> MNKTMLKIVAFGVAVIGFYMYITVYVTGLSGTGGGGTATGVSAEAGEQIFWGDGQCSTCHKIGSSGSATRGPDQEGLAERAEERAKELGLSSGLEYLVESIIDPEKYVVEGFDKIMPRVYDPPIMLSREKILAVLAYLQSLGGEPDLDAIMKFKDKIPEASKTKVKPWVPPLAVTAEEGEQVFFDESLDVTCGKCHMVNGKGQKVGPELTGIGAIQTPQYFVESILEPSAVIVKGYETVFVITADGIPYNGLIKSDTEEELTLILEESGSVEEVVIPKDEIEDMKKQEVSICPGNIGELLSVRQFYAVIEYLRSLK

Kustd1711 is a putative electron transfer protein encoded on the nitrite oxidoreductase (nxr) gene cluster of anaerobic ammonium-oxidizing (anammox) bacteria and consists of two heme-containing domains and one additional domain. Here, we describe a diheme cytochrome c with high heme redox potentials of about +350 mV, despite having a large overall negative charge, which typically reduces redox potentials. High-resolution crystal structures, spectroelectrochemical measurements, and high-end computational methods show how this is achieved: each heme iron has a calcium cation positioned next to it at a distance of only 6.9 Å, raising their redox potentials by several hundred millivolts through electrostatic interaction. We suggest that this has evolved to provide the protein with a high redox potential despite its large negative surface charge, which it likely requires for interactions with redox partners.

To improve our confidence in the assignment of the various transitions, we mutated the distal methionine ligands in both the N- and C-terminal heme sites to histidine and cysteine. To confirm that the sites can accommodate these mutations while maintaining six-coordinate heme binding and calcium binding, we determined the crystal structures of the C-terminal domain methionine mutants M292H and M292C to 1.12 and 1.70 Å resolution, respectively using the same crystallization conditions as for the wt protein, that is, including 200 mM Ca2+. This showed that these mutants are able to support both six-coordinate heme ligation as well as calcium binding, although in the M292H mutant, the plane of the distal His292’s side chain is at an angle of ∼75° with the plane of the heme porphyrin system rather than perpendicular to it. The M→C mutants did not show clearly defined transitions at low potentials and showed considerable hysteresis, which precluded meaningful fitting. That the crystal structures of the mutant showed a fully occupied calcium site in both domains is probably because of the high (200 mM) calcium concentration used in crystallization.>[2x]MGHHHHHHHHHHSSGHIDDDDKHMRGREEKAPEEPQPVKMPENNSVVEATWNDVQLEDSLGMEVGYRLIPMVDFQQDGELLGRIRSIRKKFAQDMGFLPPVVHIRDNMDLQPARYRILMKGVEIGSGDAYPGRWLAINPGTAAGTLPGEKTVDP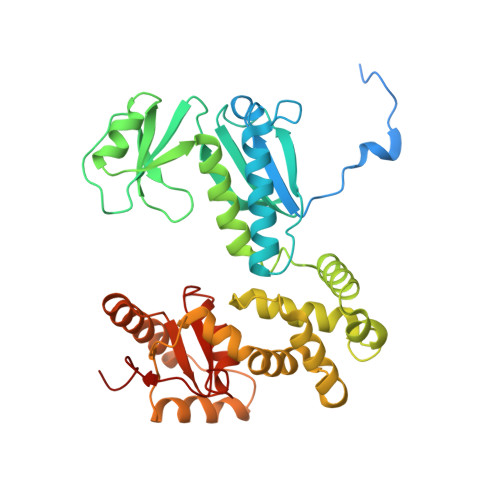AFGLDAIWIESALKEQAQIQGFTVVEASTVVATHLNHLIGQFSAELFGRQEAQQLLDRVSQEMPKLTEDLVPGVVTLTTLHKVLQNLLAEKVPIRDMRTILETLAEHAPLQSDPHELTAVVRVALGRAITQQWFPGNEEVQVIGLDTALERLLLQALQGGGGLEPGLADRLLAQTQEALSRQEMLGAPPVLLVNHALRPLLSRFLRRSLPQLVVLSNLELSDNRHIRMTATIGGK>[2x]MGTLKAIIAPSVLASNISKLAEETQRMESLGAEWIHLDVMDMHFVPNLSFGPPVINNLKKYTKSIFFDVHLMVEYPEKYVPLLKTSNQLTFHFEALNEDTERCIQLA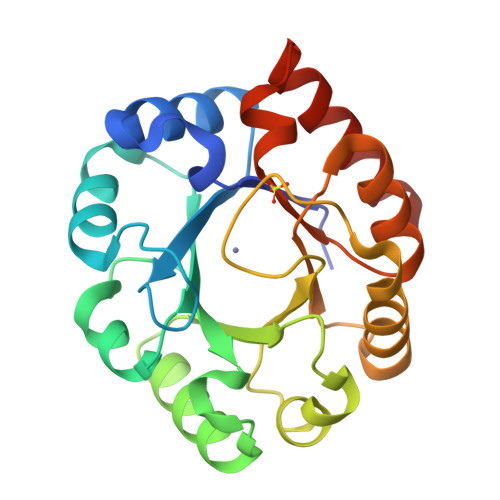KEIRDNNLWCGISIKPKTDVQKLVPILDTNLINTVLVMTVEPGFGGQSFMHDMMGKVSFLRKKYKNLNIQVDGGLNIETTEISASHGANIIVAGTSIFNAEDPKYVIDTMRVSVQKYLNN>[2x]MGGGGTDRVRRSEAITHGTPFQKAAALVDLAEDGIGLPVEILDQSSFGESARYYFIFTRLDLIWSLNYFALLFLNFFEQPLWCEKNPKPSCKDRDYYYLGELPYLTNAESIIYEVITLAILLVHTFFPISYEGSRIFWTSRLNLVKVACVVILFVDVLVDFLYLSPLAFDFLPFRIAPYVRVIIFILSIRELRDTLVLLSGMLGTYLNILALWMLFLLFASWIAFVMFENTQQGLTVFTSYGATLYQMFILFTTSNNPDVWIPAYKSSRWSSVFFVLYVLIGVYFVTNLILAVVYDSFKEQLAKQVSGMDQMKRRMLEKAFGLIDSDKNGEIDKNQCIKLFEQLTNYRTLPKISKEEFGLIFDELDD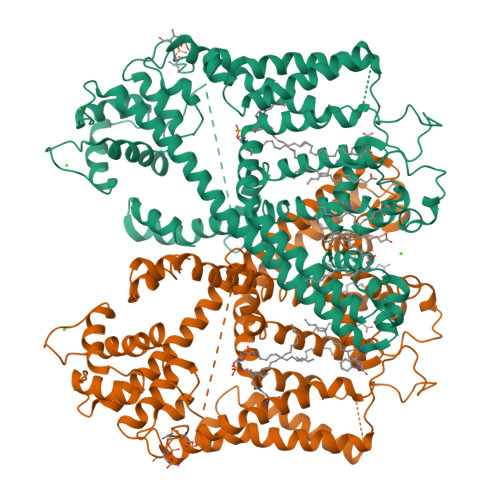TRDFKINKDEFADLCQAIALRFQKEEVPSLFEHFPQIYHSALSQQLRAFVRSPNFGYAISFILIINFIAVVVETTLNIEESSAQKPWQVAEFVFGWIYVLEMALKIYTYGFENYWREGANRFDFLVTWVIVIGETATFITPDENTFFSNGQWIRYLLLARMLRLIRLLMNVQRYRAFIATFITLIPSLMPYLGTIFCVLCIYCSIGVQVFGGLVNAGNKKLFETELAEDDYLLFNFNDYPNGMVTLFNLLVMGNWQVWMESYKDLTGTWWSITYFVSFYVITILLLLNLVVAFVLEAFFTELDLEEEEKCQGQDSQEKRNRRRSAGSKSRSQRVDTLLHHMLGDELSKPECSTSDTLVPR quinoxalin-6-amine | C8 H7 N3 | 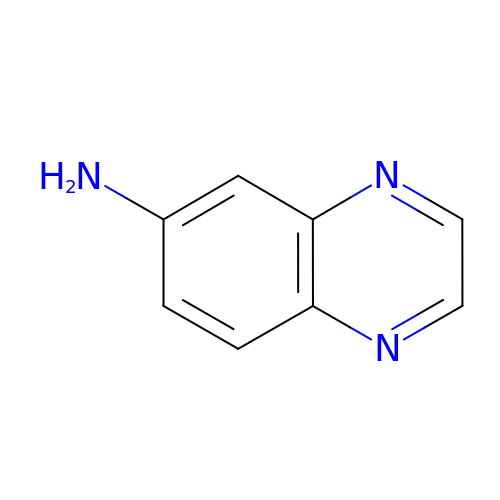MSGRFBKVMUKEGZ-UHFFFAOYSA-N> MNNQKTFKGLRLAALGLVAVAAFTAGCSDVSTELKTPVYKTKLTAEEIRNSAFKPEFPKQYASYERNDETTVMTEYKGSVPFNKNDNVNPLPEGYRHAQPYLKNLWLGYPFMYEYREARGHTYAIQDFLHIDRINRYAEKGGLPATCWNCKTPKMMEWVKESGDGFWAKDVNEFRDKIDMKDHTIGCATCHDPQTMELRITSVPLTDYLVSQGKDPKKLPRNEMRALVCGQCHVEYYFNGPTMGVNKKPVFPWAEGFDPADMYRYYDKHGDLQVKGFEGKFADWTHPASKTPMIKAQHPEYETWINGTHGAAGVTCADCHMSYTRSDDKKKISSHWWT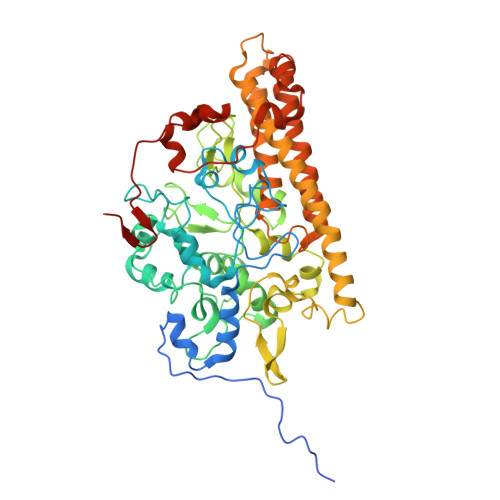SPMKDPEMRACRQCHSDKTPDYLKSRVLFTQKRTFDLLLAAQEVSVKAHEAVRLANEYQGAKAAGYDDLMIQAREMVRKGQFFWDYVSAENSVGFHNPAKALDTLAQSQQFSQKAIDLAMEATQYGIGKDLSGDIKTIVPPILKMNRKLQQDPEFMKTHKWFQYLPVLPKADQVWDGQKRLVSAKQ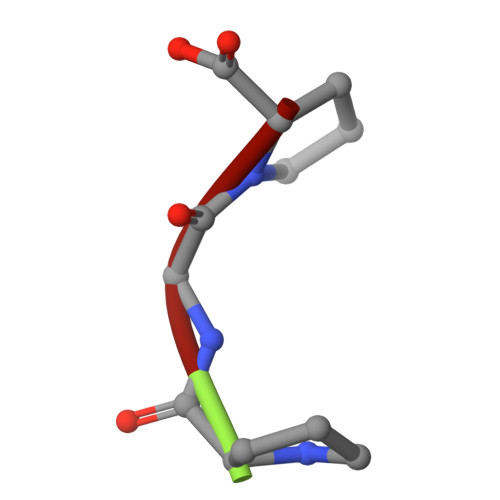> PGP> MASITSRASARASCSQANTRAGRVALSGGALLRPARPARSFVPARKQQQGAVRRGGALSARASAVEDIRKVLSDSSSPVAGQKYDYILVGGGTAACVLANRLSADGSKRVLVLEAGPDNTSRDVKIPAAITRLFRSPLDWNLFSELQEQLAERQIYMARGRLLGGSSATNATLYHRGAAGDYDAWGVEGWSSEDVLSWFVQAETNADFGPGAYHGSGGPMRVENPRYTNKQLHTAFFKAAEEVGLTPNSDFNDWSHDHAGYGTFQVMQDKGTRADMYRQYLKPVLGRRNLQVLTGAAVTKVNIDQAAGKAQALGVEFSTDGPTGERLSAELAPGGEVIMCAGAVHTPFLLKHSGVGPSAELKEFGIPVVSNLAGVGQNLQDQPACLTAAPVKEKYDGIAISDHIYNEKGQIRKRAIASYLLGGRGGLTSTGSDRGAFVRTAGQALPDLQVRFVPGMALDPDGVSTYVRFAKFQSQGLKWPSGITMQLIACRPQSTGSVGLKSADPFAPPKLSPGYLTDKDGADLATLRKGIHWARDVARSSALSEYLDGELFPGSGVVSDDQIDEYIRRSIHSSNAITGTCKMGNAGDSSSVVDNQLRVHGVEGLRVVDASVVPKIPG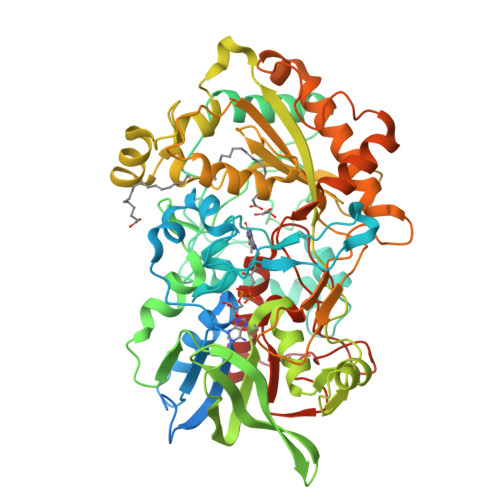GQTGAPVVMIAERAAALLTGKATIGASAAAPATVAA> AQVINTFDGVADYLQTYHKLPDNYITKSEAQALGWVASKGNLADVAPGKSIGGDIFSNREGKLPGKSGRTWREADINYTSGFRNSDRILYSSDWLIYKTTDAY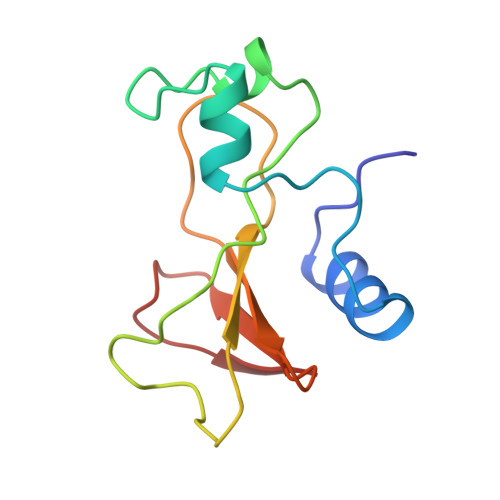QTFTKIR>[2x]SNAMKNSMTYIQLLNETLHCYASKGSLEAYTYIMEHAKGIVGNEAQIYNFKYALASAAGLEEEAMHVMKEAIIEKGF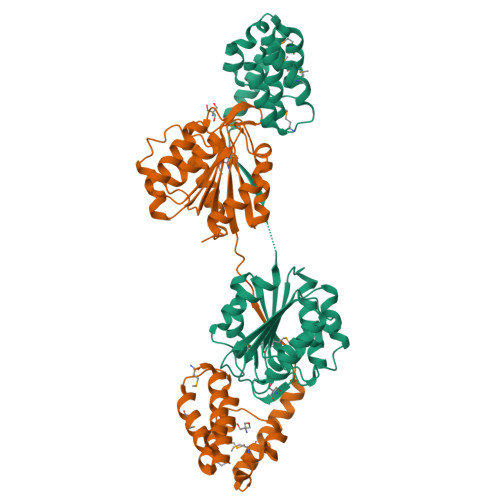WYGNEYLISDDDLKPLHKFEEFHQMVQLCKEREELAKKTERADVKYIDSKKKEKLFIAMHGDQENIAIVEPYWKSVLDQDYTLALPQSSQIQFSDGFVWDDIQRGKEELKEHYVKFIENHRGESVIIGGFSAGARVALYTILHKDIDVDGFIFMAPWLPEIDEWNELLEVLQDKNIKGYVVCGDQDEDCFECTQQFVQVLKDKNIEHEFKVVPNLKHDYPEDFDELLKEAIKYIEDKSNK> GCCSHPACAVDHPE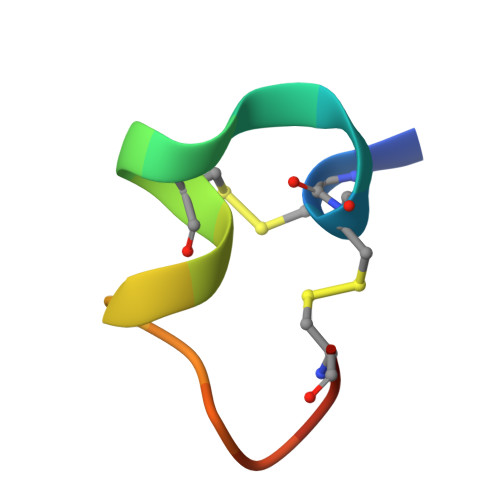ICX> MYWVRRKTIGGSGLPYTENEILEWRKEGVKRVLVLPEDWE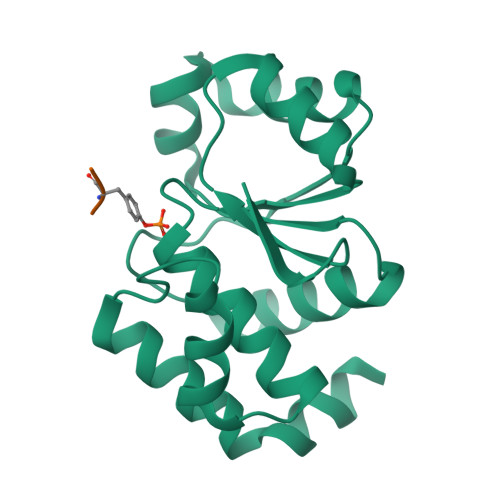IEESWGDKDYYLSILKKNGLQPLHIPIPDGGVPSDSQFLTIMKWLLSEKEGNLVHSVGGIGRTGTILASYLILTEGLEVESAIDEVRLVRPGAVQTYEQEMFLLRVEGMRKSWLKNIYSNS;> AYR~{N}-(2-chloranyl-5-phenyl-pyridin-3-yl)benzenesulfonamide 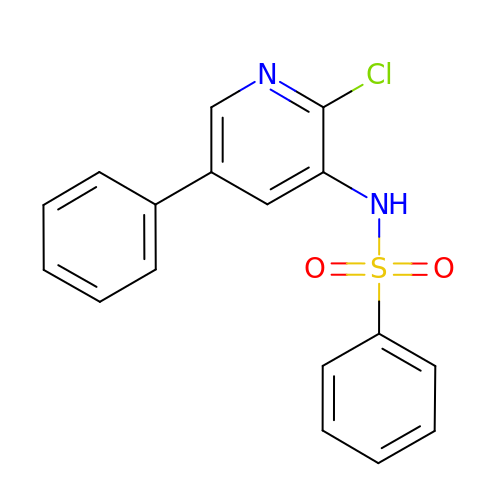| C17 H13 Cl N2 O2 S | BKSZOJANUXVKCU-UHFFFAOYSA-N(1S,3S)-N3-(5-pentan-3-ylpyrazolo[1,5-a]pyrimidin-7-yl)cyclopentane-1,3-diamine 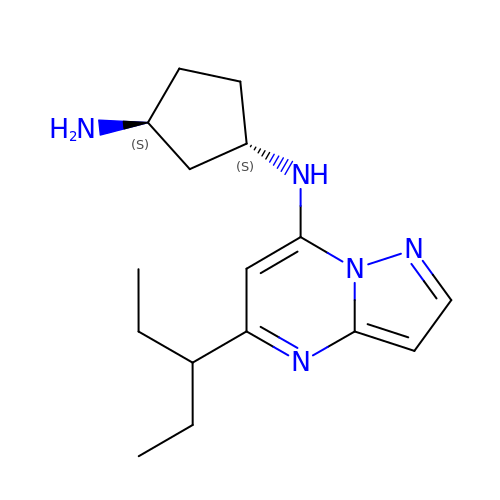| C16 H25 N5 | VYKCLMALANGCDF-UHFFFAOYSA-N> QQQSAFKQLYTELFNNEGDFSKVSSNLK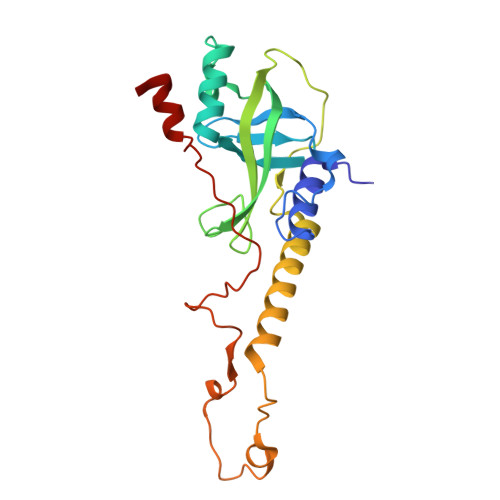KPLKCYVKESYPHFLVTDGYFFVAPYFTKEAVNEFHAKFPNVNIVDLTDKVIVINNWSLELRRVNSAEVFTSYANLEARLIVHSFKPNLQERLNPTRYPVNLFRDDEFKTTIQHFRHTALQAAINKTVKGDNLVDISKVADAAGKKGKVDAGIVKASASKGDEFSDFSFKEGNTATLKIADIFVQEKG>MRCIGISNRDFVEGVSGGSWVDIVLEHGSCVTTMAKNKPTLDFELIKTEAKQPATLRKYCIEAKLTNTTTDSRCPTQGEPSLNEEQDKRFVCKHSMVDRGWGNGCGLFGKGGIVTCAMFTCKKNMKGKVVQPENLEYTIVITPHSGEEHAVGNDTGKHGKEIKITPQSSITEAELTGYGTVTMECSPRTGLDFNEMVLLQMENKAWLVHRQWFLDLPLPWLPGADTQGSNWIQKETLVTFKNPHAKKQDVVVLGSQEGAMHTALTGATEIQMSSGNLLFTGHLKCRLRMDKLQLKGMSYSMCTGKFKVVKEIAETQHGTIVIRVQYEGDGSPCKIPFEIMDLEKRHVLGRLITVNPIVTEKDSPVNIEAEPPFGDSYIIIGVEPGQLKLNWFKKGSSIGQMIETTMRGAKRMAILGDTAWDFGSLGGVFTSIGKALHQVFGAIYGAAFSGVSWIMKILIGVIITWIGMNSRSTSLSVSLVLVGVVTLYLGVMVQA[72x];>FHLTTRNGEP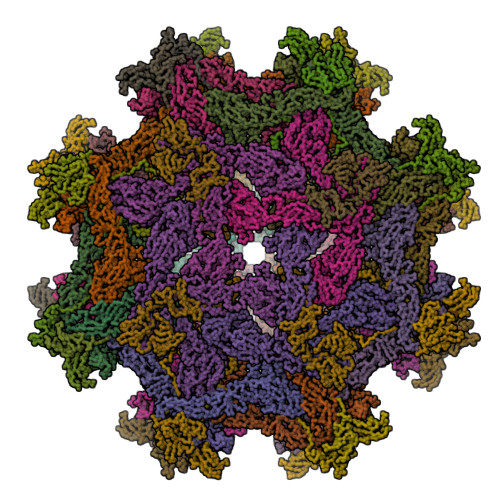HMIVSRQEKGKSLLFKTEDGVNMCTLMAMDLGELCEDTITYKCPFLKQNEPEDIDCWCNSTSTWVTYGTCTTTGEHRREKRSVALVPHVGMGLETRTETWMSSEGAWKHAQRIETWILRHPGFTIMAAILAYTIGTTHFQRALIFILLTAVAPSMT[72x]>MKTKLMTLQDATGFFRDGMTIMVGGFMGIGTPSRLVEALLESGVRDLTLIANDTAFVDTGIGPLIVNGRVRKVIASHIGTNPETGRRMISGEMDVVLVPQGTLIEQIRCGGAGLGGFLTPTGVGTVVEEGKQTLTLDGKTWLLERPLRADLALIRAHRCDTLGNLTYQLSARNF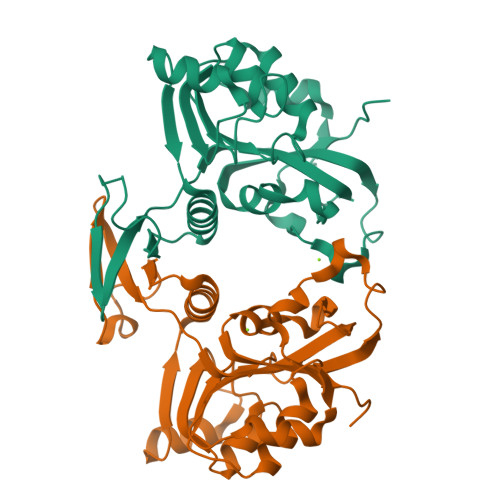NPLIALAADITLVEPDELVETGELQPDHIVTPGAVIDHIIVSQESK[2x]>[4x]STKTNVVEVLNKQVANWNVLYVKLHNYHWYVTGPHFFTLHEKFEEFYNEAGTYIDELAERILALEGKPLATMKEYLATSSVNEGTSKESAEEMVQTLVNDYSALIQELKEG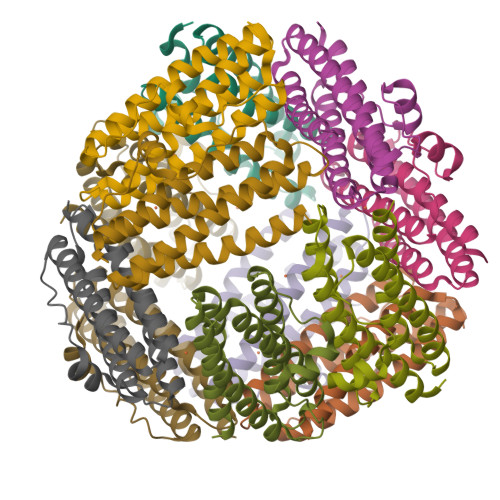MEVAGEAGDATSADMLLAIHTTLEQHVWMLSAFLK>[4x]GSVHKHTGRNCGRKFKIGEPLYRCHECGCDDTCVLCIHCFNPKDHVNHHVCT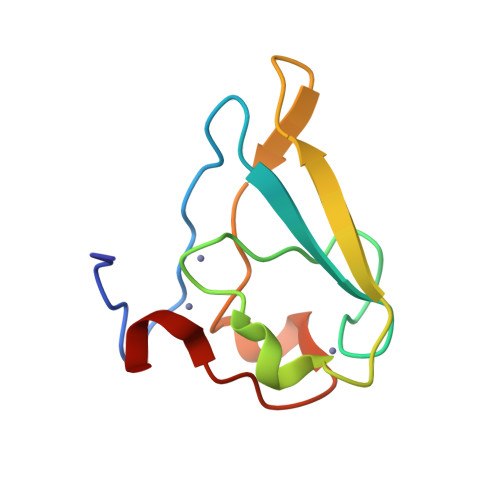DICTEFTSGICDCGDEEAWNSPLHCKAEEQ;> RDAA>[2x]QAKHKQRKRLKSSCKRHPLYVDFSDVGWNDWIVAPPGYHAFYCHGECPFPLADHLNST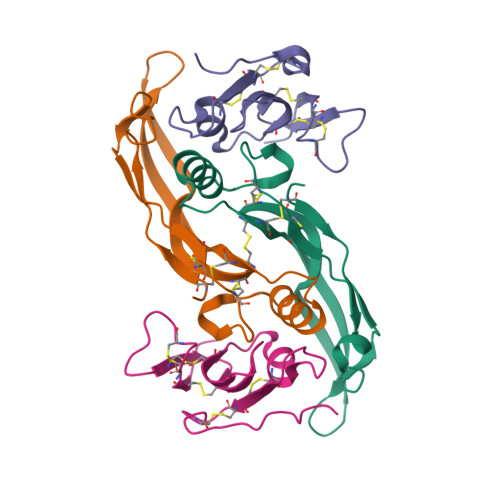NHAIVQTLVNSVNSKIPKACCVPTELSAISMLYLDENEKVVLKNYQDMVVEGCGCR;>GSGAMAQNLDSMLHGTGMKSDSDQKKSENGVTLAPEDTLPFLKCYCSGHCPDDAINNTCITNGHCFAIIEEDDQGETTLASGCMKYEGSDFQCKDSPKAQLRRTIECCRTNLCNQYLQPTLPPVVIGPFFDGSIR[2x]>[4x]GSARPSSSMADFRKFFAKAKHIVIISGAGVSAESGVPTFRGAGGYWRKWQAQDLATPLAFAHNPSRVWEFYHYRRE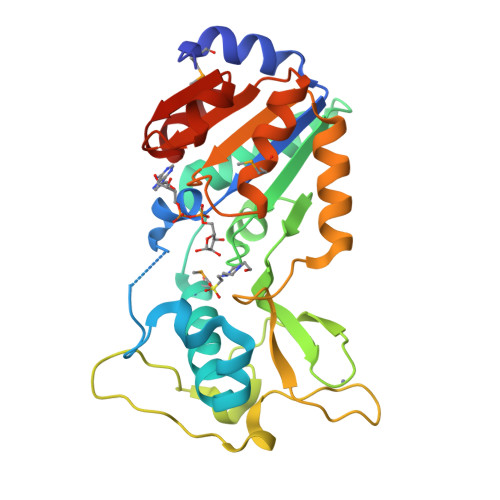VMGSKEPNAGHRAIAECETRLGKQGRRVVVITQNIDELHRKAGTKNLLEIHGSLFKTRCTSCGVVAENYKSPICPALSGKGAPEPGTQDASIPVEKLPRCEEAGCGGLLRPHVVWFGENLDPAILEEVDRELAHCDLCLVVGTSSVVYPAAMFAPQVAARGVPVAEFNTETTPATNRFRFHFQGPCGTTLPEALA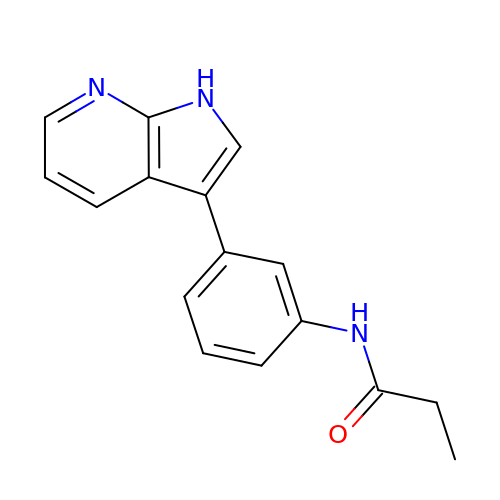~{N}-[3-(1~{H}-pyrrolo[2,3-b]pyridin-3-yl)phenyl]propanamide | C16 H15 N3 O | CXHYISUBNJBKTE-UHFFFAOYSA-N> GSRMSGNNMSTPLPAIVPAARKATAAVIFLHGLGDTGHGWAEAFAGIRSSHIKYICPHAPVRPVTLNMNVAMPSWFDIIGLSPDSQEDESG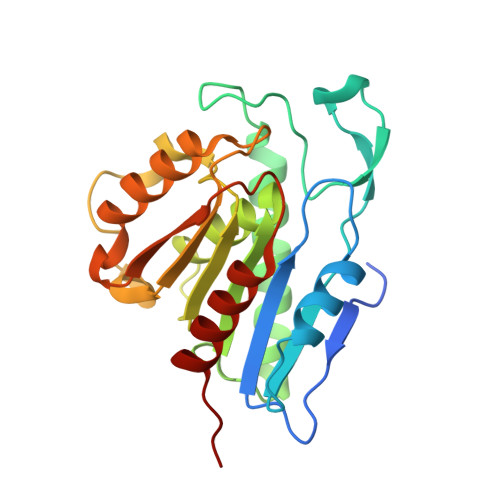IKQAAENIKALIDQEVKNGIPSNRIILGGFSQGGALSLYTALTTQQKLAGVTALSCWLPLRASFPQGPIGGANRDISILQCHGDCDPLVPLMFGSLTVEKLKTLVNPANVTFKTYEGMMHSSCQQEMMDVKQFIDKLLPPID> DPISNAIENAVSTLADTTISRVTAANTAASSHSLGTGRVPALQAAETGASSNASDENLIETRCVMNRNGVNEASVEHFYSRAGLVGVVEVKDSGTSQDGYTVWPIDVMGFVQQRRKLELSTYMRFDAEFTFVSNLNDSTTPGMLLQYMYVPPGAPKPDGRKSYQWQTATNPSIFAKLSDPPPQVSVPFMSPASAYQWFYDGYPTFGEHKQATNLQYGQCPNNMMGHFAIRTVSESTTGKNVHVRVYMRIKHVRAWVPRPFRSQAYMVKNYPTYSQTISNTAADRASITTTDYEGGVPANPQRTF;> SPSVEACGYSDRVAQLTVGNSTITTQEAANIVLSYGEWPGYCPSTDATAVDKPTRPDVSVNRFYTLSTKSWKTESTGWYWKFPDVLNDTGVFGQNAQFHYLYRSGFCMHVQCNASKFHQGALLVVVIPEFVVAASSPATKPNGQGLYPDFAHTNPGKEGQVFRDPYVLDAGIPLSQALVFPHQWINLRTNNCATIIMPYVNALPFDSALNHSNFGLAVIPISPLKYCNGATTEVPITLTIAPLNSEFSGLRQAIKQ;> GLPTELKPGTNQFLTTDDGT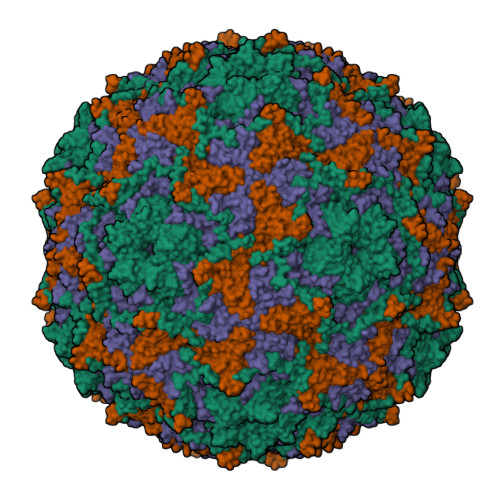SPPILPGFEPTPLIHIPGEFTSLLDLCRIETILEVNNTTGTTGVNRLLIPVRAQNNVDQLCASFQVDPGRNGPWQSTMVGQICRYYTQWSGSLKVTFMFTGSFMATGKMLIAYTPPGSAQPTTREAAMLGTHIVWDFGLQSSVTLVIPWISNTHFRAVKTGGVYDYYATGIVTIWYQTNFVVPPDTPSEANIIALGAAQENFTLKLCKDTDEIRQTAEYQN;> GAQVSAQKSGTHETGNIATEGSTINFTNINYYKDSYAASASRQDFTQDPTKFTSPVLDAIKEAAAPLQ>[2x]MAAQNEQRPERIKTTPYLEGDVLSSDSGPLLSVFALQEIMQKVRQVQADYMTATREVDFTVPDVQQILDDIKALAAEQVYKIVKVPSTSFRHIVTQSRDRVLRVDTYYEEMSQVGDVITEDEPEKFYSTIIKKVRFIRGKGSFILHDIPARDHRGMEVAEPEVLGVEFKNVLPVLTAEHRAMIQNALDGSIIENGNVATRDVDVFIGACSEPIYRIYNRLQGYIEAVQLQELRNSIGWLERLGQRKRITYSQEVLTDFRRQDMIWVLALQLPVNPQVVWDVPRSSIANLIMNIATCLPTGEYIAPNPRISSITLTQRITTTGPFAILTGSTPTAQQLNDVRKIYLALMFPGQIILDLKIDPGERMDPAVRMVAGVVGHLLFTAGGRFTNLTQNMARQLDIALNDYLLYMYNTRVQVNYGPTGEPLDFQIGRNQYDCNVFRADFATGTGYNGWATIDVEYRDPAPYVHAQRYIRYCGIDSRELINPTTYGIGMTYHCYNEMLRMLVAAGKDSEAAYFRSMLPFHMVRFARINQIINEDLHSVFSLPDDMFNALLPDLIAGAHQNADPVVLDVSWISLWFAFNRSFEPTHRNEMLEIAPLIESVYASELSVMKVDMRHLSLMQRRFPDVLIQARPSHFWKAVLNDSPEAVKAVMNLSHSHNFINIRDMMRWVLLPSLQPSLKLVLEEEAWAAANDFEDLMLTDQVYMHRDMLPEPRLDDIERFRQEGFYYTNMLEAPPEIDRVVQYTYEIARLQANMGQFRAALRRIM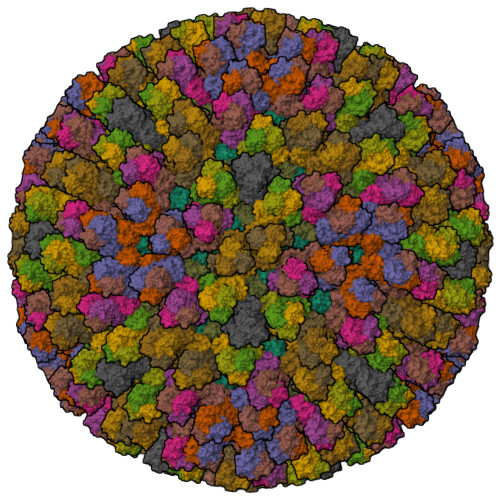DDDDWVRFGGVLRTVRVKFFDARPPDDILQGLPFSYDTNEKGGLSYATIKYATETTIFYLIYNVEFSNTPDSLVLINPTYTMTKVFINKRIVERVRVGQILAVLNRRFVAYKGKMRIMDITQSLKMGTKLAAPTV;>MDTIAARALTVMRACATLQEARIVLEANVMEILGIAINRYNGLTLRGVTMRPTSLAQRNEMFFMCLDMMLSAAGINVGPISPDYTQHMATIGVLATPEIPFTTEAANEIARVTGETSTWGPARQPYGFFLETEETFQPGRWFMRAAQAATAVVCGPDMIQVSLNAGARGDVQQIFQGRNDPMMIYLVWRRIENFAMAQGNSQQTQAGVTVSVGGVDMRAGRIIAWDGQAALHVRNPTQQNAMVQIQVVFYISMDKTLNQYPALTAEIFNVYSFRDHTWHGLRTAIRNRTTLPNMLPPIFPPNDRDSILTLLLLSTLADVYTVLRPEFAMHGVNPMPGPLTAAIARAAYV[13x]>[9x]MAQILPIRFQEHLQLQNLGINPANIGFSTLTMESDKFICIREKVGEQAQVVIIDMNDPSNPIRRPISADSAIMNPASKVIALKAGKTLQIFNIEMKSKMKAHTMTDDVTFWKWISLNTVALVTDNAVYHWSMEGESQPVKMFDRHSSLAGCQIINYRTDAKQKWLLLTGISAQQNRVVGAMQLYSVDRKVSQPIEGHAASFAQFKMEGNAEESTLFCFAVRGQAGGKLHIIEVGTPPTGNQPFPKKAVDVFFPPEAQNDFPVAMQISEKHDVVFLITKYGYIHLYDLETGTCIYMNRISGETIFVTAPHEATAGIIGVNRKGQVLSVCVEEENIIPYITNVLQNPDLALRMAVRNNLAGAEELFARKFNALFAQGNYSEAAKVAANAPKGILRTPDTIRRFQSVPAQPGQTSPLLQYFGILLDQGQLNKYESLEL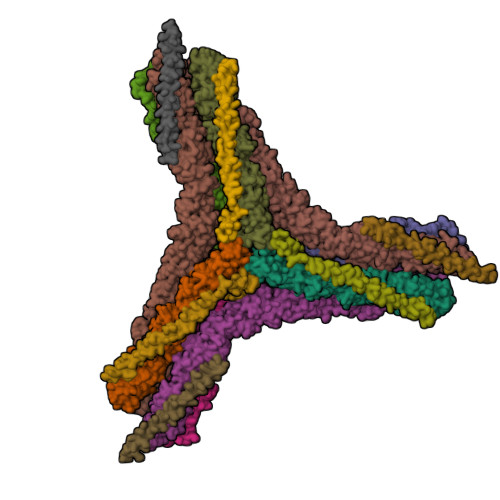CRPVLQQGRKQLLEKWLKEDKLECSEELGDLVKSVDPTLALSVYLRANVPNKVIQCFAETGQVQKIVLYAKKVGYTPDWIFLLRNVMRISPDQGQQFAQMLVQDEEPLADITQIVDVFMEYNLIQQCTAFLLDALKNNRPSEGPLQTRLLEMNLMHAPQVADAILGNQMFTHYDRAHIAQLCEKAGLLQRALEHFTDLYDIKRAVVHTHLLNPEWLVNYFGSLSVEDSLECLRAMLSANIRQNLQICVQVASKYHEQLSTQSLIELFESFKSFEGLFYFLGSIVNFSQDPDVHFKYIQAACKTGQIKEVERICRESNCYDPERVKNFLKEAKLTDQLPLIIVCDRFDFVHDLVLYLYRNNLQKYIEIYVQKVNPSRLPVVIGGLLDVDCSEDVIKNLILVVRGQFSTDELVAEVEKRNRLKLLLPWLEARIHEGCEEPATHNALAKIYIDSNNNPERFLRENPYYDSRVVGKYCEKRDPHLACVAYERGQCDLELINVCNENSLFKSLSRYLVRRKDPELWGSVLLESNPYRRPLIDQVVQTALSETQDPEEVSVTVKAFMTADLPNELIELLEKIVLDNSVFSEHRNLQNLLILTAIKADRTRVMEYINRLDNYDAPDIANIAISNELFEEAFAIFRKFDVNTSAVQVLIEHIGNLDRAYEFAERCNEPAVWSQLAKAQLQKGMVKEAIDSYIKADDPSSYMEVVQAANTSGNWEELVKYLQMARKKARESYVETELIFALAKTNRLAELEEFINGPNNAHIQQVGDRCYDEKMYDAAKLLYNNVSNFGRLASTLVHLGEYQAAVDGARKANSTRTWKEVCFACVDGKEFRLAQMCGLHIVVHADELEELINYYQDRGYFEELITMLEAALGLERAHMGMFTELAILYSKFKPQKMREHLELFWSRVNIPKVLRAAEQAHLWAELVFLYDKYEEYDNAIITMMNHPTDAWKEGQFKDIITKVANVELYYRAIQFYLEFKPLLLNDLLMVLSPRLDHTRAVNYFSKVKQLPLVKPYLRSVQNHNNKSVNESLNNLFITEEDYQALRTSIDAYDNFDNISLAQRLEKHELIEFRRIAAYLFKGNNRWKQSVELCKKDSLYKDAMQYASESKDTELAEELLQWFLQEEKRECFGACLFTCYDLLRPDVVLETAWRHNIMDFAMPYFIQVMKEYLTKVDKLDASESLRKEEEQATETQPIVYGQPQLMLTAGPSVAVPPQAPFGYGYTAPAYGQPQPGFGYSM;>[6x]MADDFGFFSSSESGAPEAAEEDPAAAFLAQQESEIAGIENDEGFGAPAGSQGGLAQPGPASGASEDMGATVNGDVFQEANGPADGYAAIAQADRLTQEPESIRKWREEQRKRLQELDAASKVMEQEWREKAKKDLEEWNQRQSEQVEKNKINNRIADKAFYQQPDADIIGYVASEEAFVKESKEETPGTEWEKVAQLCDFNPKSSKQCKDVSRLRSVLMSLKQTPLSR> MLKMEAVPLRLEHRQEVIDIIVASFYNKADLEQWLKPGVLRTDYSDILNDIWNVLVERDLSFVVYDTNTDRIIGTALNFDARNEP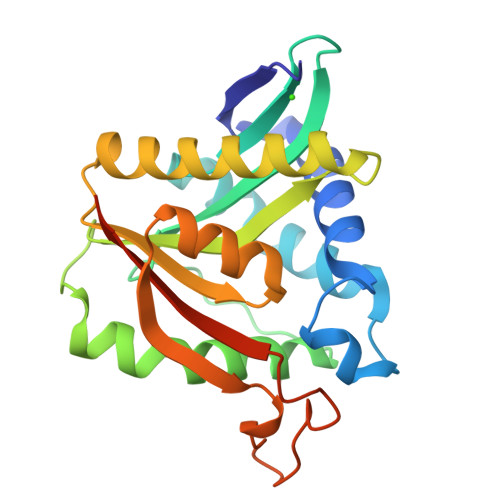EVDIKSKLLIVFEFLEFCEGPIRDNYLPKGLNQILHSFMMGTAEKLNPRENIACMHFMEHEVLRVAREKQFAGIFTTNTSPLTQQLADVYHYKTLLNFQVNEYVHSDGSRPFGDAPDEQRAIVHWKEVGKGSHHHHHH Maf (for multicopy associated filamentation) proteins represent a large family of conserved proteins implicated in cell division arrest but whose biochemical activity remains unknown. Here, we show that the prokaryotic and eukaryotic Maf proteins exhibit nucleotide pyrophosphatase activity against 5-methyl-UTP, pseudo-UTP, 5-methyl-CTP, and 7-methyl-GTP, which represent the most abundant modified bases in all organisms, as well as against canonical nucleotides dTTP, UTP, and CTP. The protomer structures of the four Maf proteins revealed a large β sheet containing seven β strands (β1 to β7) with two α-helical subdomains on one side and one long α helix on another side. Thus, pyrophosphatase activity of Maf proteins toward canonical and modified nucleotides might provide the molecular mechanism for a dual role of these proteins in cell division arrest and house cleaning.

In many eukaryotic Maf proteins, including the human ASMTL, the N-terminal YhdE-like Maf domain is covalently fused to another domain encoding a predicted methyltransferase protein, whereas in some archaeal genomes (e.g., Staphylothermus marinus), the Maf gene is associated with a methyltransferase gene, suggesting a functional relationship between these proteins. Whereas both YceF-like proteins were inactive against these substrates (30–90 nmol/min per milligram of protein), the four YhdE-like Maf proteins (E. coli YhdE, BSU28050, YOR111W, and ASMTL-Maf) showed significant metal-dependent pyrophosphatase activity against pyrimidine nucleoside triphosphates dTTP, UTP, and CTP. In the ASMTL-Maf structure, two protomers form a dimer via the formation of a common large β sheet through the interaction between their β6 strands. This oligomeric state is consistent with the results of our gel-filtration analysis, which showed that ASMTL-Maf exists as a dimer in solution (observed molecular mass, 44.5 kDa; predicted monomer molecular mass, 28.3 kDa), whereas YhdE exists as a mixture of dimers and tetramers (observed molecular mass, 47.2 and 101 kDa, respectively; predicted monomer molecular mass, 24 kDa) and YceF as a mixture of monomers and dimers (observed molecular mass, 24.8 and 50 kDa, respectively; predicted molecular mass, 24.5 kDa). In ASMTL-Maf, the phosphate molecule is located close to the side chains of the conserved Ser19 (2.4 Å), Arg24 (2.6 Å), Lys65 (2.6 Å), and Lys100 (4.0 Å), and it probably mimics the position of the substrate γ-phosphate. In Maf proteins and structurally similar ITP pyrophosphatases, the side chain of the predicted catalytic Asp (ASMTL-Maf Asp88; YOR111W Asp103) interacts with the conserved Lys (ASMTL-Maf Lys65, 2.9 Å; YOR111W Lys74), possibly stabilizing the unprotonated state of Asp.

>[2x]LLHKRVVLASASPRRQEILSNAGLRFEVVPSKFKEKLDKASFATPYGYAMETAKQKALEVANRLYQKDLRAPDVVIGADTIVTVGGLILEKPVDKQDAYRMLSRLSGREHSVFTGVAIVHCSSKDHQLDTRVSEFYEETKVKFSELSEELLWEYVHSGEPMDKAGGYGIQALGGMLVESVHGDFLNVVGFPLNHFCKQLVKLYYPPRPEDLRRSVKHDSIPAADTFEDLS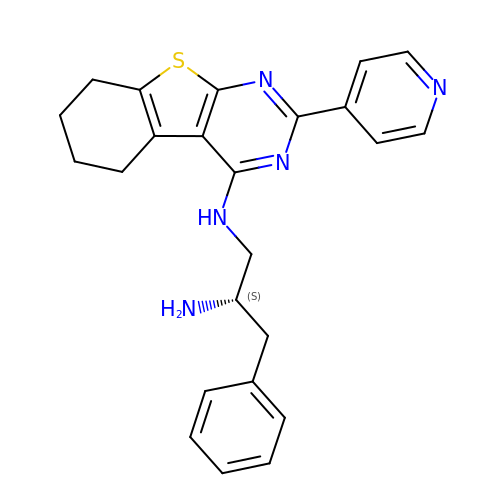(2S)-3-phenyl-N~1~-[2-(pyridin-4-yl)-5,6,7,8-tetrahydro[1]benzothieno[2,3-d]pyrimidin-4-yl]propane-1,2-diamine | C24 H25 N5 S | NRHASZRDWOUMFD-SFHVURJKSA-N>SNAVDSLLDSVKWDNKGLAVAIAQNVDTGAILMQGFANREAVATTISSRKATFYSRSRSSLWTKGETSNNFINVHDVFLDCDRDSIIYLGKPDGPTCHTGAETCYYTPVFDLLKEEEVEGNKLALTSLYALESTISQRKAEVVEENGKPSWTKRLLLNDKLLCSKIREEANELCETLENNEDKSRTASEMADVLYHAMVL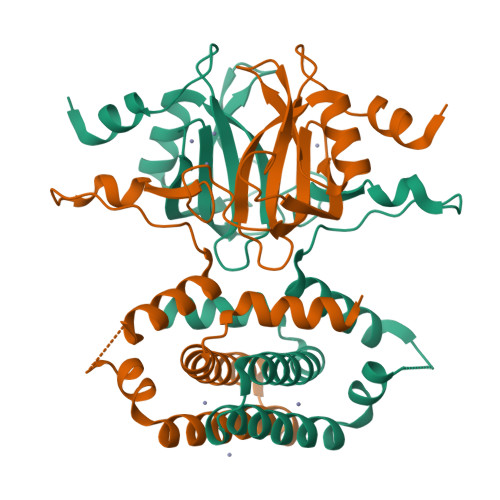LALKDVKVEEVLQVLRQRFSKSGIEEKRSRPTQKSVEN[2x]>[2x]VVTAQWVPRVDIKEEVNHFVLYADLPGIDPS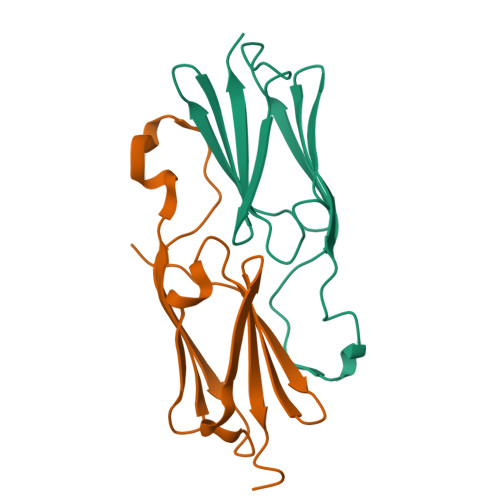QIEVQMDKGILSIRGERKSESSTETERFSRIERRYGSFHRRFALPDSADADGITAAGRNGVLEIRIPKRPAA> MEGMDPLAVLAESRLLPLLTVRGGEDLLGLARVLEEEGVGALEITLRTEKGLEALKALRKSGLLLGAGTVRSPKEA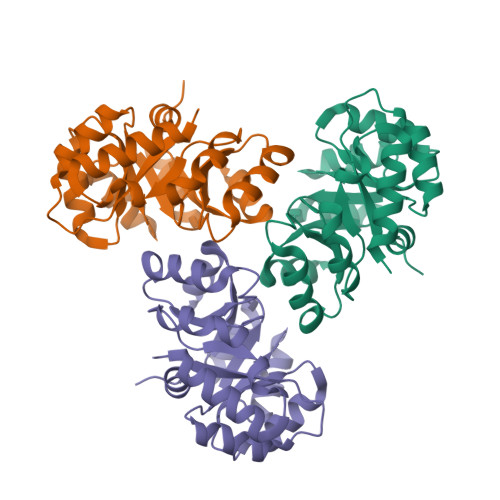EAALEAGAAFLVSPGLLEEVAALAQARGVPYLPGVLTPTEVERALALGLSALKFFPAEPFQGVRVLRAYAEVFPEVRFLPTGGIKEEHLPHYAALPNLLAVGGSWLLQGNLEAVRAKVRAAKALLSPQAPG> GDHPTFNKITPNLAEFAFSLYRQLAHQSNSTNILFSPVSIAAAFAMLSLGAKGDTHDEIL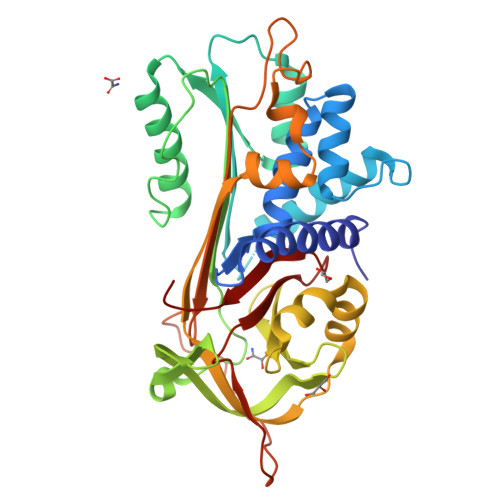EGLNFNLTEIPEAQIHEGFQELLRTLNQPDSQLQLTTGNGLFLSEGLKLVDKFLEDVKKLYHSEAFTVNFGDTEEAKKQINDYVEKGTQGKIVDLVKELDRDTVFALVNYIFFKGKWERPFEVKDTEEEDFHVDQVTTVKVPMMKRLGMFNIQHSKKLSSWVLLMKYLGNATAIFFLPDEGKLQHLENELTHDIITKFLENEDRRSASLHLPKLSITGTYDLKSVLGQLGITKVFSNGADLSGVTEEAPLKLSKAVHKAVLTIDEKGTEAAGAMFLEAIPMSIPPEVKFNKPFVFLIIEQNTKAPLFMGRVVNPTQK> YAAAT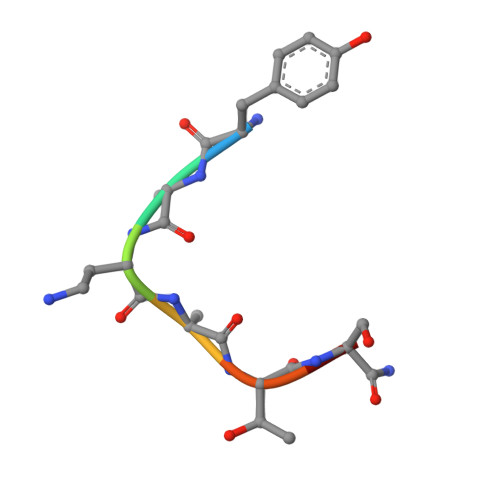SA1-(piperidin-4-yl)-1,6-dihydroimidazo[4,5-d]pyrrolo[2,3-b]pyridine | C13 H15 N5 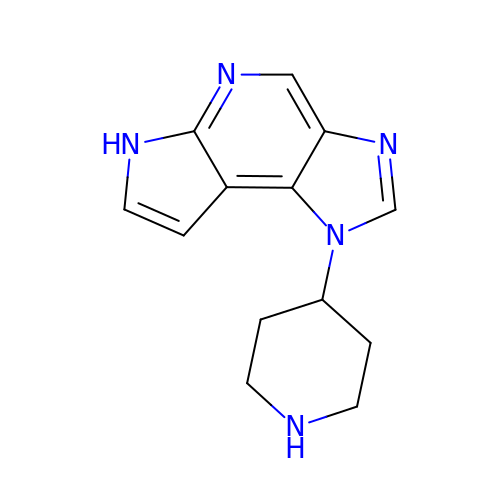| VTICMARMQUNXBS-UHFFFAOYSA-N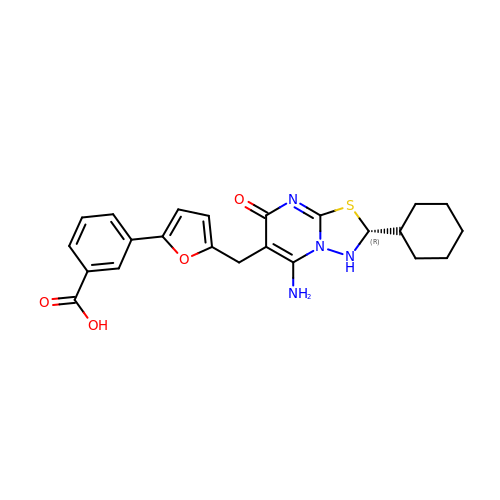3-(5-{[(2R)-5-amino-2-cyclohexyl-7-oxo-2,3-dihydro-7H-[1,3,4]thiadiazolo[3,2-a]pyrimidin-6-yl]methyl}furan-2-yl)benzoic acid | C23 H24 N4 O4 S | HSMUYTKNVZBPLA-OAQYLSRUSA-N>GAMNPDPEATMDRSLLQRQDLPYRFSAVDLDSVDGQRHYRLWLGRPLQAPPAAGYPVVWMLDGNAAVGALDESTLRRLADGDAPLLVAIGYRTPLRIDRAGRTFDYTPASPGQADQRDPLNGLPSGGADAFLDLLRDGMRPAVAAQAPLDTARQTLWGHAYGGLLVLHALFTRPGEFARYAAASPSLWWRDGAILGERAGLEQRLRGKRAELLLWRGSAEPASPRGSLKAEPGQAMARLVDDLRRVAGLTLDFQPLDGLGHG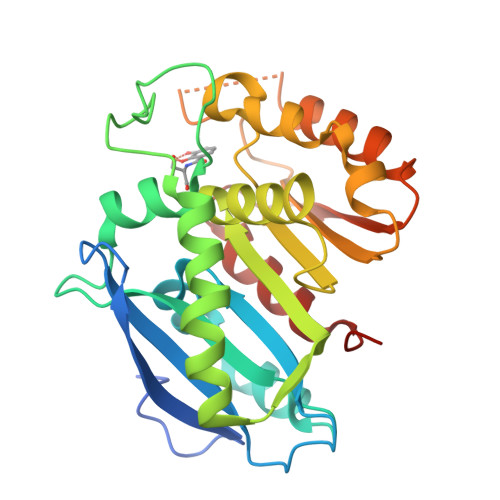ETLGASLRLLLARPAVERQR[2x]>[2x]GMFPGVWRKHHPDVD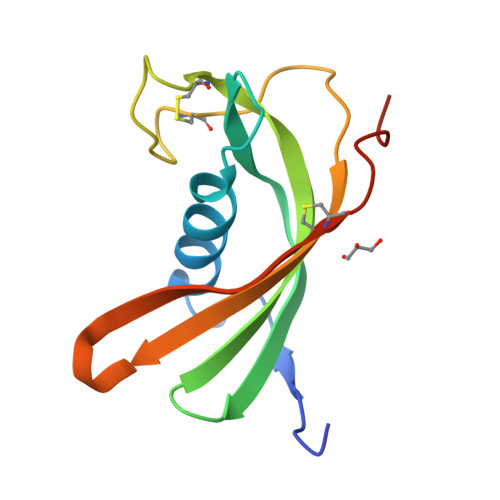PRYKEWAHFAISSQVENRTNFDTLMTLISVESQVIAGVDYKLKMKVAESTCVIGVDSYSKERCYLKVNVPYMLCTAVVNYMPWEHKTILKSYDCSDRVYGVKSAE> MDVPGPVSRRAAAAAATVLLRTARVRRECWFLPTALLCAYGFFASLRPSEP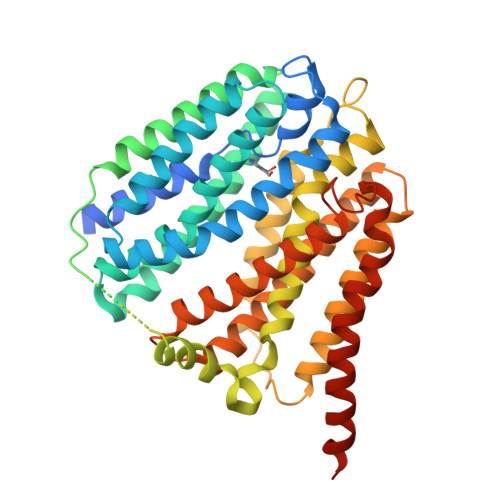FLTPYLLGPDKNLTEREVFNEIYPVWTYSYLVLLFPVFLATDYLRYKPVVLLQGLSLIVTWFMLLYAQGLLAIQFLEFFYGIATATEIAYYSYIYSVVDLGMYQKVTSYCRSATLVGFTVGSVLGQILVSVAGWSLFSLNVISLTCVSVAFAVAWFLPMPQKSLFFHHIPSTCQRVNGIKVQNGGIVTDTPASNHLPGWEDIESKIPLNMEEPPVEEPEPKPDRLLVLKVLWNDFLMCYSSRPLLCWSVWWALSTCGYFQVVNYTQGLWEKVMPSRYAAIYNGGVEAVSTLLGAVAVFAVGYIKISWSTWGEMTLSLFSLLIAAAVYIMDTVGNIWVCYASYVVFRIIYMLLITIATFQIAANLSMERYALVFGVNTFIALALQTLLTLIVVDASGLGLEITTQFLIYASYFALIAVVFLASGAVSVMKKCRKLEDPQSSSQVTTS>MDLKVEIETLYEVSKILSSSLNLETTVPYIFRLLKKLMGFERLTLTIYDPSTDQIVVRATSSGKFPKEGFKKGEGITGKVWKHGVPIVIPDISQEPEFLNKVWKRKKSKKKIAFIAVPIKSGGKVIGVLSADKEINEKDSLDEYTRFLSMIATLIANS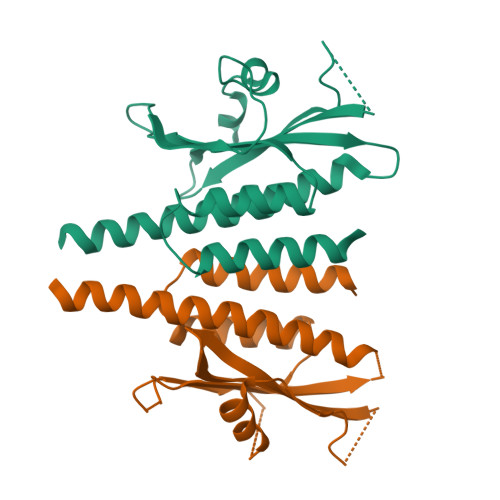FSLERKVQAERKSLEEE[2x]> MNKFREWITFSVISCLVAVTLVGCDKPEEQREEAPAREVDVLSVKTEPFTVFAELPGRIEPVRVAEVRARVAGIVLKRTFEEGADVKAGDVLFQIDPAPFKAALSRAQGELARAEAQLFQAQAMVRRYEPLVKIDAVSQQDFDNAMAALQSAQADKRSAQANVETARLDLGYAEVRAPIAGRIGRAQVT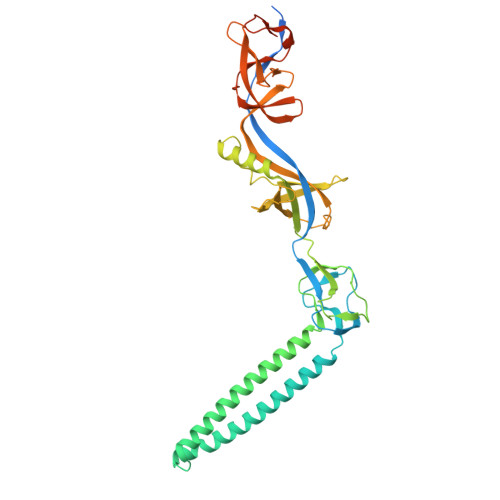EGALVGQGEATLLARIQQLDPVYADFTQPAADALRLRAAIAEGKVAGASDQPLSLRVDGTDIERKGTLLFTDISVDRSTGQIALRGQFDNPEGVLLPGMYVRVRTPQGLNQNAILVPQRAVQRSADGQASVMLLGEGDTVEVRQVTTGAMQGSRWQISEGLQAGDKVITSSLAAIRPGAKVIPREQGAAEKAPQSQAQWSHPQFEK>[2x]MTIRSYKNLNLVRANIETESRQFIENKNYSIQSIGPMPGSRAGLRVVFTRPGVNLATVDIFYNGDGSTTIQYLTGANRSLGQELADHLFETINPAEFEQVNMVLQGFVETSVLPVLELSADESHIEFREHSRNAHTVVWKIISTSYQDELTVSLHITTGKLQIQGRPLSCYRVFTFNLAALLDLQGLEKVL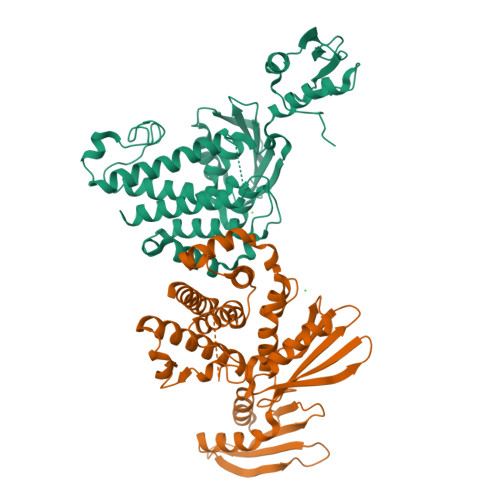IRQEDGKANIVQQEVARTYLQTVMADAYPHLHVTAEKLLVSGLCVKLAAPDLPDYCMLLYPELRTIEGVLKSKMSGLGMPVQQPAGFGTYFDKPAAHYILKPQFAATLRPEQINIISTAYTFFNVERHSLFHMETVVDASRMISDMARLMGKATRAWGIIKDLYIV>SMMPIVNVKLLEGRSDEQLKNL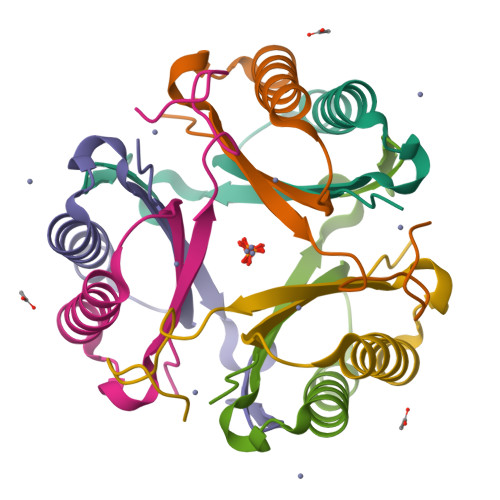VSEVTDAVEKTTGANRQAIHVVIEEMKPNHYGVAGVRKSDQ[2x]> GGUCUCUCUGGUUAAGCCAGAUCUGAGCC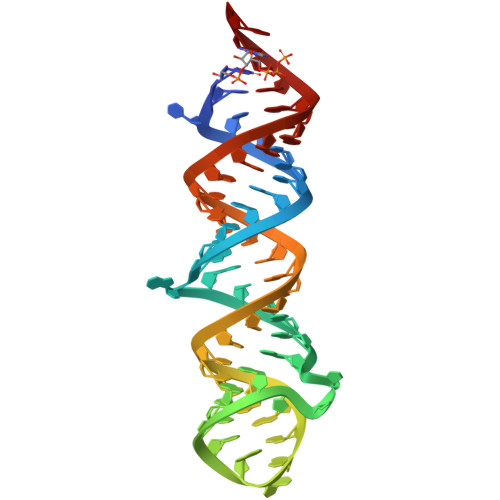GAAAAGCUCUCUGGCUAACUAGGGAACCA> MSLLLTIAKEYKRLCQDAKAAQMMTVGTVSNYTTFKKWTTSRKEKNPSLRMRWAMSSKFPIIANKRMLEEAQIPKEHNNVALWEDTEDVSKRDHVLASASCINYWNFCGPCVNNSEVIKEVYKSRFGRLERRKEIMWKELRFTLVDRQRRRVDTQPVEQRLRTGEIKDLQMWTLFEDEAPLASKFILDNYGLVKEMRSKFANKPLNKEVVAHMLEKQFNPESRFLPVFGAIRPERMELIHALGGETWIQEANTAGISNVDQRKNDIRAVCRKVCLAANASIMNAKSKLVEYIKSTSMRIGETERKLEELILETDDVSPEVTLCKSALGGQLGKTLSFGPMLLKKISGSGVKVKDTVYIQGVRAVQFEYWSEQEEFYGEYKSATALFSRKERSLEWITIGGGINEDRKRLLAMCMIFCRDGDYFKDAPATITMADLSTKLGREIPYQYVMMNWIQKSEDNLEALLYSRGIVETNPGKMGSSMGIDGSKRAIKSLRAVTIQSGKIDMPESKEK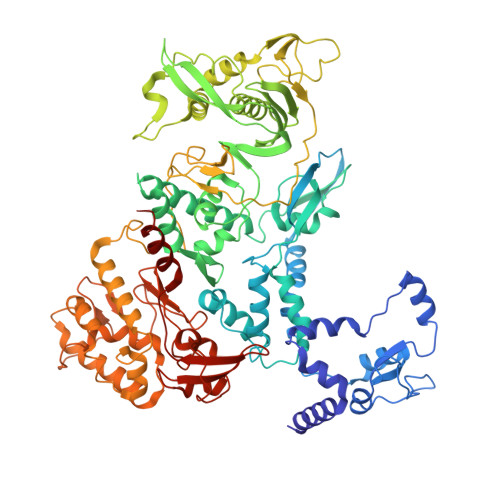IHLELSDNLEAFDSSGRIVATILDLPSDKKVTFQDVSFQHPDLAVLRDEKTAITKGYEALIKRLGTGDNDIPSLIAKKDYLSLYNLPEVKLMAPLIRPNRKGVYSRVARKLVSTQVTTGHYSLHELIKVLPFTYFAPKQGMFEGRLFFSNDSFVEPGVNNNVFSWSKADSSKIYCHGIAIRVPLVVGDEHMDTSLALLEGFSVCENDPRAPMVTRQDLIDVGFGQKVRLFVGQGSVRTFKRTASQRAASSDVNKNVKKIKMSN>MTVVPENFVPGLDGVVAFTTEIAEPDKDGGALRYRGVDIEDLVSQRVTFGDVWALLVDGNFGSGLPPAEPFPLPI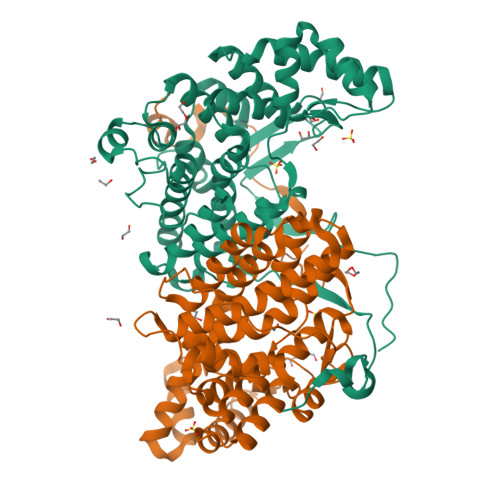HSGDVRVDVQAGLAMLAPIWGYAPLLDIDDATARQQLARASVMALSYVAQSARGIYQPAVPQRIIDECSTVTAEFMTRWQGEPDPRHIEAIDAYWVSAAEHGMNASTFTARVIASTGADVAAALSGAIGAMSGPLHGGAPARVLPMLDEVERAGDARSVVKGILDRGEKLMGFGHRVYRAEDPRARVLRAAAERLGAPRYEVAVAVEQAALSELRERRPDRAIETNVEFWAAVVLDFARVPANMMPAMFTCGRTAGWCAHILEQKRLGKLVRPSAIYVGPGPRSPESVDGWERVLTTAHHHHHH[8x]> EAEFQYFGSYYCQPGRDVIVHLFEWKWTDIERECQWLADHNYCGVQVSPPNEHRIVTDPPYPWWQRYQPVSYTMNSRSGSETQFRNMVTTCNNLGVYIYVDGVLNHMTGGGSGTGSDGNSFDGDSLQYPGVPYGPNDFHGSDDCSTSDGEIHDYNNPTEVRNCRLSGLRDLDGSANYVRDVEAEFANRLIGWGVAGFRLDACKHMWPGDLEAILGRLNQLNTQWFPAGRNAYIYQQVIDLGGEAVKATEYTYLGRVTEFKHGQNLGNVVRKNNGQRLANLVNFGEGWGQLSGFDALVFIDNHDNQRGHGAGGFGTILTFFEANMYKIATAFELAWDYGHVRLMSSYNWPRNIVNGVDTNDWVGPPTNGGGDTKDVECFNGEWICEHRWREMYNMVRFHNVAIGNPVSNWWDNGFQAIAFGRGNRGFIFINNEDFAITQTLQTGLPGGEYCDVISCDNNRPPCGNSGGACRATVI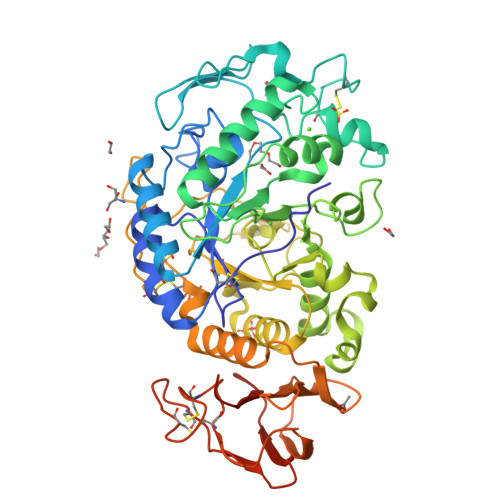VNGDGTATFDVPNGENPMIAIHVFLEQKLISEEDLNSAVDHHHHHH>[4x]APQLHHHHHHDLYENLYFQGKLDPASKSRSCGEVRQIYGAKGFSLSDVPQAEISGEHLRICPQGYTCCTSEMEEN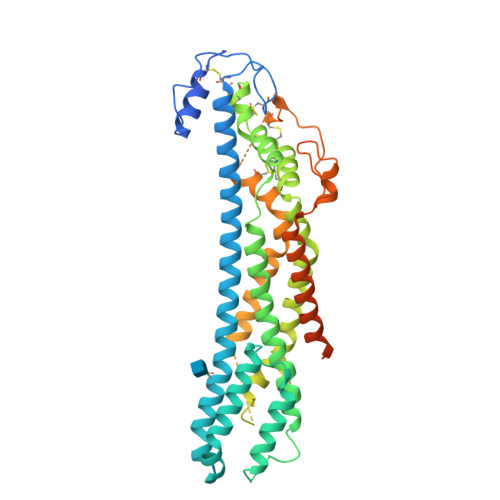LANRSHAELETALRDSSRVLQAMLATQLRSFDDHFQHLLNDSERTLQATFPGAFGELYTQNARAFRDLYSELRLYYRGANLHLEETLAEFWARLLERLFKQLHPQLLLPDDYLDCLGKQAEALRPFGEAPRELRLRATRAFVAARSFVQGLGVASDVVRKVAQVPLGPECSRAVMKLVYCAHCLGVPGARPCPDYCRNVLKGCLANQADLDAEWRNLLDSMVLITDKFWGTSGVESVIGSVHTWLAEAINALQDNRDTLTAKVIQGCGNPKVNPQGPGPEEKRRRGKLAPRERPPSGTLEKLVSEAKAQLRDVQDFWISLPGTLCSEKMALSTASDDRCWNGMARGRYLPEVMGDGLANQINNPEVEVDITKPDMTIRQQIMQLKIMTNRLRSAYNGNDVDFQDASDDGSGSGSGDGCLDDLCSRKVSRKSSSSRTPLTHALPGLSEQEGQKT>[2x]RTFDLEE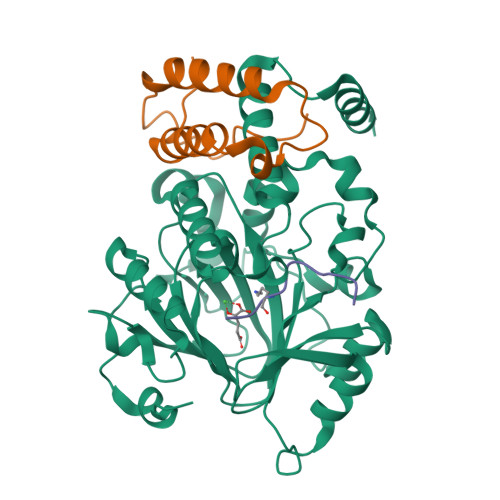KLQTNKYNANFVTFMEGKDFNVEYIQRGGLRDPLIFKNSDGLGIKMPDPDFTVNDVKMCVGSRRMVDVMDVNTQKGIEMTMAQWTRYYETPEEEREKLYNVISLEFSHTRLENMVQRPSTVDFIDWVDNMWPRHLKESQTESTNAILEMQYPKVQKYCLMSVRGCYTDFHVDFGGTSVWYHIHQGGKVFWLIPPTAHNLELYENWLLSGKQGDIFLGDRVSDCQRIELKQGYTFVIPSGWIHAVYTPTDTLVFGGNFLHSFNIPMQLKIYSIEDRTRVPNKFRYPFYYEMCWYVLERYVYCITNRSHLTKDFQKESLSMDME;>[2x]QVHLTHFELEGLRCLVDKLESLPLHKKCVPTGIEDEDALIADVKILLEELASSDPKLALTGVPIVQWP;>APATGGVKKPHRYRP[2x]> AATTGYDAVDDLLHYHERGNGIQINGKDSFSNEQAGLFITRENQTWNGYKVFGQPVKLTFSFPDYKFSSTNVAGDTGLSKFSAEQQQQAKLSLQSWADVANITFTEVAAGQKANITFGNYSQDRPGHYDYGTQAYAFLPNTIWQGQDLGGQTWYNVNQSNVKHPATEDYGRQTFTHEIGHALGLSHPGDYNAGEGNPTYNDVTYAEDTRQFSLMSYWSETNTGGDNGGHYAAAPLLDDIAAIQHLYGANLSTRTGDTVYGFNSNTGRDFLSTTSNSQKVIFAAWDAGGNDTFDFSGYTANQRINLNEKSFSDVGGLKGNVSIAAGVTIENAIGGSGNDVIVGNAANNVLKGGAGNDVLFGGGGADELWGGAGKDIFVFSAASDSAPGASDWIRDFQKGIDKIDLSFFNKEANSSDFIHFVDHFSGTAGEALLSYNASSNVTDLSVNIGGHQAPDFLVKIVGQVD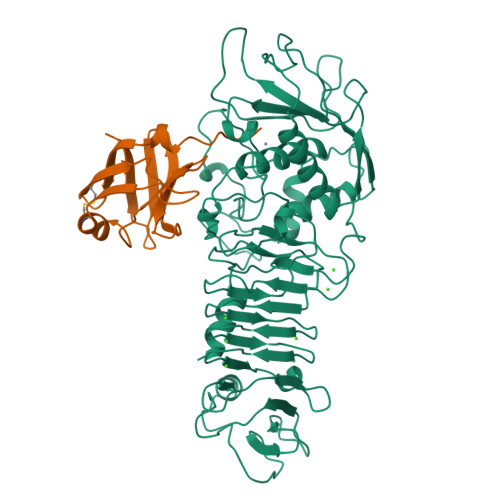VATDFIV;> SSLRLPSAAELSGQWVLSGAEQHCDIRLNTDVLDGTTWKLAGDTACLQKLLPEAPVGWRPTPDGLTLTQADGSAVAFFSRNRDRYEHKLVDGSVRTLKKKA> GPGLKQKIVIKVAMEGNNCRSKAMALVASTGGVDSVALVGDL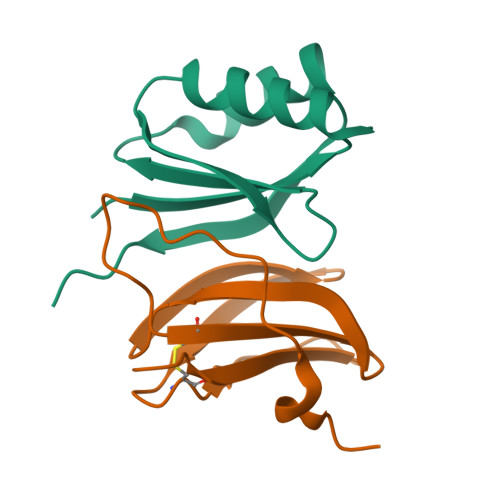RDKIEVVGYGIDPIKLISALRKKVGDAELLQVSQAKED;> METGNKYIEKRAIDLSRERDPNFFDHPGIPVPECFWFMFKNNVRQDAGTCYSSWKMDMKVGPNWVHIKSDDNCNLSGDFPPGWIVLGKKRPGF>[2x]MASHHHHHHGSMAEGEEYDKILVLNFGSQYFHLIVKRLNNIKIFSETKDYGVELKDIKDMNIKGVILSGGPYSVTEAGSPHLKKEVFEYFLEKKIPIFGICYGMQEIAVQMNGEVKKSKTSEYGCTDVNILRNDNINNITYCRNFGDSSSAMDLYSNYKLMNETCCLFENIKSDITTVWMNHNDEVTKIPENFYLVSSSENCLICSIYNKEYNIYGVQYHPEVYESLDGELMFYNFAYNICKCKKQFDP

GMP synthesis proceeds through two steps, the first being the conversion of IMP to xanthine monophosphate (XMP) catalysed by IMP dehydrogenase followed by GMPS (guanosine 5′-monophosphate synthetase; EC 6.3.5.2) converting XMP to GMP4. GMPS is a class-I (trpG-type) amidotransferase in which the catalytic reaction occurs in two physically distant domains, a GATase (glutamine amidotransferase) domain and an ATPPase (ATP pyrophosphatase) domain5. Hydrolysis of glutamine to glutamate and ammonia occurs in the GATase domain, whereas formation of the intermediate AMP-XMP from ATP and XMP occurs in the ATPPase domain. Ammonia generated in the GATase domain attacks the intermediate to generate GMP.

We purified and crystallized PfGMPS, PfGMPS_C89A and PfGATase, and solved their structures by molecular replacement to resolutions of 3.6, 3.15 and 2.6 Å, respectively. The GATase segment displays an α/β-structure of nine β-strands surrounded by five α-helixes. Compared with Hs- and EcGMPS, the PfGMPS GATase domain exhibits an extension (119–151) inserted between β5 and β6. This unique insertion lacks even in other Plasmodium GMPS and its role is yet to be determined. The structure of the isolated PfGATase domain is similar to those in the full-length PfGMPS_C89A/Gln and PfGMPS wild-type with root mean square deviations (RMSDs) of 0.67 and 1.37 Å. Size-exclusion chromatography shows that in solution PfGATase is largely monomeric while PfATPPase is dimeric, confirming that dimerization is mediated via this latter domain. PfGATase exhibited leaky glutaminase activity, unlike other GMPS characterized to date1116 but similar to PfGMPS. Although PfGATase alone has very-poor affinity for glutamine, the high specific activity values support (as seen in the structure) that the triad and oxyanion hole are positioned in the conformation required for catalysis and the loop movement occurring upon ligand-binding to ATPPase primarily leads to increase in substrate affinity. Interestingly, when superposing the structures of individual GATase domains (PfGATase, PfGMPS_C89A/Gln, PfGMPS) no conformational differences were observed, inferring that the major determinant for an increased glutamine-affinity in the presence of ATP and XMP should be found in the ATPPase domain close to the interface.>MGPSVLLLLALLVGFVLLLVRGYPKARGHLPPGPRPLPLLGNLLQMDRGGFLNSFMRIREKYGDVFTVHLGPRPVVMLYGTEAIREALVDQAEAFSGRGTIAVIKPVIGDYGMIFSNGERWKVLRRFSLATMRDFGMGKRSVEDRIQEEAQCLVEELQKSQGAPLDPTFLFQCITANIICSIVFGERYDYKDRQFLRLLDLFYRTFSLMSSFSSQVFELFSGFMKYFPGAHRQITRNLQEILDYVGQSVEKHRATLDPSNPRDFIDTYLLRMEKEKSNQHTEFHHQNLLISVLSLFFAGTETTSTTLRYGFLLMLKYPHVAEKVQKEIDQVIGSHRLPTL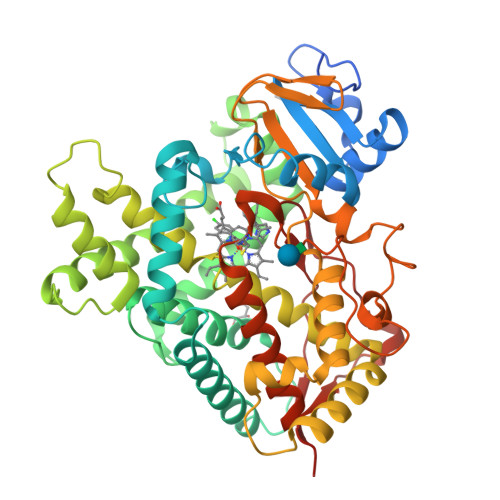EDRTKMPYTDAVIHEIQRFSDLAPIGAPHKVTKDTLFRGYLLPKNTEVYPILSSALHDPQYFEQPGTFNPDHFLDANGALKKSEAFMPFSIGKRICLGEGIARNELFLFFTTILQNFSVSSSVAPKDIDLSPKESGIGKVPQTYQISFLARHH[6x]> GHMTHYKFYEANVETNQVLVFLHGFLSDSRTYHNHIEKFTDNYHVITIDLPGHGEDQSSMDETWNFDYITTLLDRILDKYKDKSITLFGYSMGGRVALYYAINGHIPISNLILESTSPGIKEEANQLERRLVDDARAKVLDIAGIELFVNDWEKLPLFQSQLELPVEIQHQIRQQRLSQSPHKMAKALRDYGTGQMPNLWPRLKEIKVPTLILAGEYDEKFVQIAKKMANLIPNSKCKLISATGHTIHVEDSDEFDTMILGFLKEEQND

Menaquinone, vitamin K2, is a lipid soluble quinone used by bacteria for electron transport. We turn our attention now to MenH, the enzyme which catalyzes the third step in this pathway, a 2,5-elimination of pyruvate from 2-succinyl-5-enolpyruvyl-6-hydroxy-3-cyclohexadiene-1-carboxylate (SEPHCHC) to produce 2-succinyl-6-hydroxy-2,4-cyclohexadiene-1-carboxylate (SHCHC). Rigorous biochemical analysis then proved that MenH is actually responsible for the elimination of the pyruvate side chain (E.C. 4.2.99.20) and that previous studies had been compromised by the inherent reactivity of SEPHCHC, which slowly decomposes to SHCHC and pyruvate. The high-resolution crystal structure of SaMenH, an α/β hydrolase, has been determined and detailed comparisons carried out with proteins of related fold.

The enzyme crystallizes in the monoclinic space group C2 with one molecule in the asymmetric unit and diffraction data to better than 2 Å were measured in-house. At the end of the refinement there was continuous electron density for the entire polypeptide chain, residues 1-266, missing only the Gly-His residues that remain at the N-terminus following proteolytic cleavage of the histidine tag. Approximately 65% of the SaMenH residues are in well-defined elements of secondary structure. These comprise 7 β-strands and 11 α-helices arranged in the α/β hydrolase fold, a central β-sheet with a marked twist, sandwiched between α-helices. Helices α1 and α11 lie in the concave face of the β-sheet and α4 to α8 form an insertion in the canonical α/β hydrolase fold to create a domain that caps the active site. However, in SaMenH the core β-sheet consists of only seven strands due to the absence of the N-terminal strand observed in other family members. SaMenH behaves as a monomer in solution, as indicated by size-exclusion chromatography (data not shown). The residues that form the SaMenH catalytic triad, Ser89, Asp216 and His243 are positioned on one side of a water-filled tunnel formed between the cap and core domains. In SaMenH the main chain amides of Met90 and Phe23 are well placed to form the oxyanion hole; indeed a well-ordered water molecule is observed within hydrogen bonding distance of both nitrogen atoms in addition to the side chain of Ser89. The active site has a pronounced hydrophobic patch created by Trp150, Phe156, Leu153, Leu155 and Phe219, and in addition Phe23 and Leu186 (not shown) help form the base of the site. There are six basic residues in the active site (Arg93, Arg127, Arg134, Arg174, Lys218 and the catalytic His243) and a single acidic residue, Asp131.> MDVVVRLPDVAVPGEAVQASARQAVIHLVDIAGITSS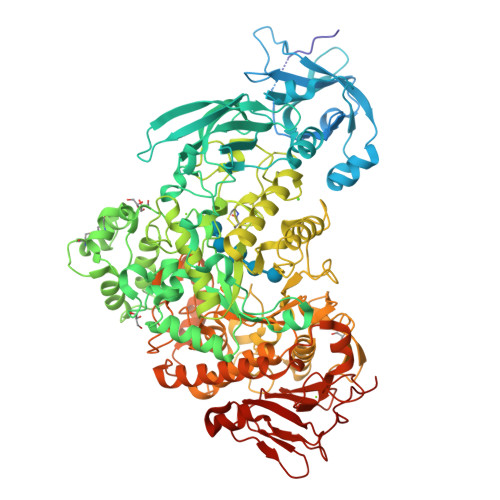TPADYATKNLYLWNNETCDALSAPVADWNDVSTTPTGSDKYGPYWVIPLTKESGCINVIVRDGTNKLIDSDLRVSFSDFTDRTVSVIAGNSAVYDSRADAFRAAFGVALADAHWVDKTTLLWPGGENKPIVRLYYSHSSKVAADSNGEFSDKYVKLTPTTVSQQVSMRFPHLASYPAFKLPDDVNVDELLQGETVAIAAESDGILSSATQVQTAGVLDDTYAAAAEALSYGAQLTDSGVTFRVWAPTAQQVELVIYSADKKVIASHPMTRDSASGAWSWQGGSDLKGAFYRYAMTVYHPQSRKVEQYEVTDPYAHSLSTNSEYSQVVDLNDSALKPEGWDGLTMPHAQKTKADLAKMTIHESHIRDLSAWDQTVPAELRGKYLALTAQESNMVQHLKQLSASGVTHIELLPVFDLATVNEFSDKVADIQQPFSRLCEVNSAVKSSEFAGYCDSGSTVEEVLTQLKQNDSKDNPQVQALNTLVAQTDSYNWGYDPFHYTVPEGSYATDPEGTARIKEFRTMIQAIKQDLGMNVIMDVVYNHTNAAGPTDRTSVLDKIVPWYYQRLNETTGSVESATCCSDSAPEHRMFAKLIADSLAVWTTDYKIDGFRFDLMLYHPKAQILSAWERIKALNPDIYFFGEGWDSNQSDRFEIASQINLKGTGIGTFSDRLRDAVRGGGPFDSGDALRQNQGVGSGAGVLPNELTTLSDDQARHLADLTRLGMAGNLADFVLIDKDGAVKRGSEIDYNGAPGGYAADPTEVVNYVSKHDNQTLWDMISYKAAQEADLDTRVRMQAVSLATVMLGQGIAFDQQGSELLRSKSFTRDSYDSGDWFNRVDYSLQDNNYNVGMPRSSDDGSNYDIIARVKDAVATPGETELKQMTAFYQELTALRKSSPLFTLGDGATVMKRVDFRNTGADQQTGLLVMTIDDGMQAGASLDSRVDGIVVAINAAPESRTLQDFAGTSLQLSAIQQAAGDRSLASGVQVAADGSVTLPAWSVAVLELPQGESQGAGLPVSSK> VWNCERITISHRKQTMAKQPGLDFQSAKGGLGELKRRLLFVIGALIVFRIGSFIPIPGIDAAVLAKLLEQQRGTIIEMFNMFSGGALSRASIFALGIMPYISASIIIQLLTVVHPTLAEIKKEGESGRRKISQYTRYGTLVLAIFQSIGIATGLPNMPGMQGLVINPGFAFYFTAVVSLVTGTMFLMWLGEQITERGIGNG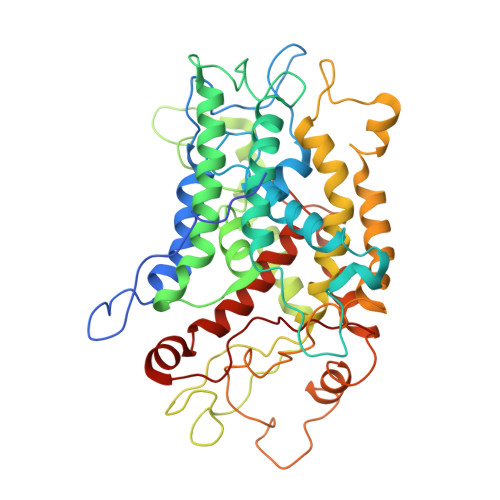ISIIIFAGIVAGLPPAIAHTIEQARQGDLHFLVLLLVAVLVFAVTFFVVFVERGQRRIVVNYAKRQQGRRVYAAQSTHLPLKVNMAGVIPAIFASSIILFPATIASWFGGGTGWNWLTTISLYLQPGQPLYVLLYASAIIFFCFFYTALVFNPRETADNLKKSGAFVPGIRPGEQTAKYIDKVMTRLTLVGALYITFICLIPEFMRDAMKVPFYFGGTSLLIVVVVIMDFMAQVQTLMMSSQYESALKKANLKGYGR~{N}-[(2~{S})-1-[[(2~{S})-2,3-dimethylbutyl]amino]-4-methyl-1-oxidanylidene-pentan-2-yl]-(phenylmethoxycarbonylaminomethyl)phosphonamidic 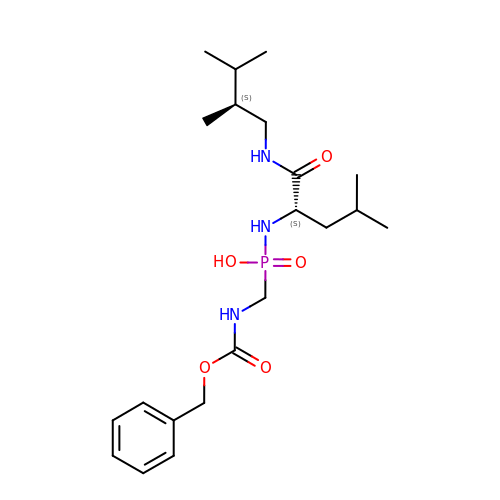acid | C21 H36 N3 O5 P | JBYBUNCIQMPTHL-MJGOQNOKSA-N FleQ and FleN act as master regulators of both flagellar motility and biofilm formation, while using different transcription activation mechanisms dependent on the target promoter and the presence or absence of the second messenger cyclic diguanylate (c-di-GMP). FleQ belongs to the NtrC subfamily of bacterial enhancer binding proteins (bEBP) and has conserved FleQ/FlrA/FlaK/FlgR homologs in Vibrio cholerae, Vibrio parahaemolyticus, Vibrio alginolyticus, Shewanella putrefaciens, and Helicobacter pylori, among others. The protein comprises an N-terminal receiver-like FleQ domain (FleQREC) and a C-terminal helix-turn-helix DNA-binding motif (FleQHTH). In between is a central bilobal AAA+ ATPase domain (FleQAAA+) composed of an N-proximal α/β subdomain (SD1) and a C-proximal α-helical SD2 module.

Due to higher protein yields and increased complex stability determined empirically, we chose again the FleND48A variant for FleN and an HTH-truncated construct for otherwise wild-type FleQ (FleQREC-AAA+). Importantly, the resulting 3D reconstruction features the same FleQAAA+-hugged FleN dimer as observed crystallographically and by cryo-EM in the absence of c-di-GMP, indicating that dinucleotide-sensing effects are mostly determined by the conformational and functional plasticity of FleQ itself. First, the global architecture of the complex is asymmetric with a 2:3 FleN:FleQ stoichiometry and overall increased flexibility. One of the FleN protomers is bound to a single FleQ subunit with reduced occupancy, resulting in slight distortion of the electron density map and loss of signal for the N-terminal receiver domain. The other FleN protomer is bound to a dimer of c-di-GMP-complexed FleQ subunits, in a conformation drastically different from the previously captured crystalline state. Whereas FleN remains bound to the nonhydrolysable AppCp, c-di-GMP is bound as a single intercalated dimer at the interface between the dimerizing FleQ protomers, i.e., in a 1:1 c-di-GMP:AAA+ stoichiometry as opposed to the 2:1 stoichiometry observed in the crystals. C-di-GMP occupies an almost identical pocket and is coordinated primarily by several arginine (backbone and side-chain interactions with R138, R144, R185, and R334 in cis and R151 in trans) and glutamate (Glu330 in cis and Glu332 in trans) residues, whereas the REC-to-AAA+ domain linker inserts deep into the ATP-binding pocket to then thread onto the surface of the interacting FleN protomer. Perhaps most surprisingly, rather than engage in an elongated symmetrical dimer as in the crystal structure, the second FleQAAA+ module establishes asymmetric tail-to-tail contacts again mediated by SD2 and the loop preceding SD1 α6.

>GPMGSKQMGSMHPVQVIAVTGGKGGVGKTNVSVNLALALADLGRRVMLLDAALGLANVDVLLGLTPKRTLADVIEGRCELRDVLLLGPGGVRIVPAASGTQSMVHLSPMQHAGLIQAFSDISDNLDVLVVDTAAGIGDSVVSFVRAAQEVLLVVCDEPTSITDAYALIKLLNRDHGMTRFRVLANMAHSPQEGRNLFAKLTKVTDRFLDVALQYVGVIPYDESVRKAVQKQRAVYEAFPRSKASLAFKAVAQKVDSWPLPANPRGHLEFFVERLVQHPATGSAV[2x];>MGSWRETKLLLIDDNLDRSRDLAVILNFLGEDQLTCNSEDWREVAAGLSNSREALCVLLGSVESKGGAVELLKQLASWDEYLPILLIGEPAPADWPEELRRRVLASLEMPPSYNKLLDSLHRAQVYREMYDQARERGRSREPNLFRSLVGTSRAIQQVRQMMQQVADTDASVLILGESGTGKEVVARNLHYHSKRREGPFVPVNCGAIPAELLESELFGHEKGAFTGAITSRAGRFELANGGTLFLDEIGDMPLPMQVKLLRVLQERTFERVGSNKTQNVDVRIIAATHKNLEKMIEDGTFREDLYYRLNVFPIEMAPLRERVEDIALLLNELISRMEHEKRGSIRFNSAAIMSLCRHDWPGNVRELANLVERLAIMHPYGVIGVGELPKKFRHVD[3x]> MHHHHHHENLYFQGPKPPIDLVVTETTATSVTLTWDSGNSEPVTYYGIQYRAAGTEGPFQEVDGVATTRYSIGGLSPFSEYAFRVLAVNSIGRGPPSEAVRARTGEQAPSSPPRRVQARMLSASTMLVQWEPPEEPNGLVRGYRVYYTPDSRRPPNAWHKHNTDAGLLTTVGSLLPGITYSLRVLAFTAVGDGPPSPTIQVKTQQGVPAQPADFQAEVESDTRIQLSWLLPPQERIIMYELVYWAAEDEDQQHKVTFDPTSSYTLEDLKPDTLYRFQLAARSDMGVGVFTPTIEARTAQSTPSAPPQKVMCVSMGSTTVRVSWVPPPADSRNGVITQYSVAYEAVDGEDRGRHVVDGISREHS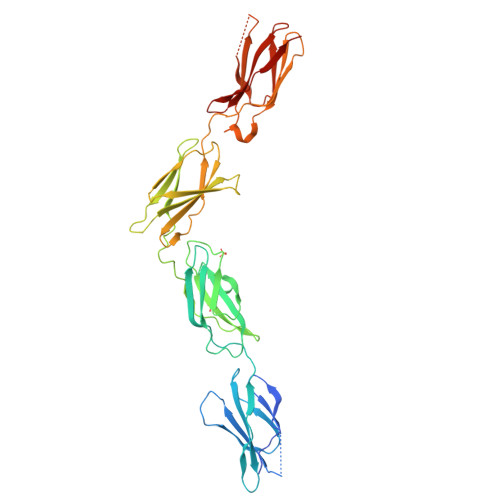SWDLVGLEKWTEYRVWVRAHTDVGPGPESSPVLVRTDED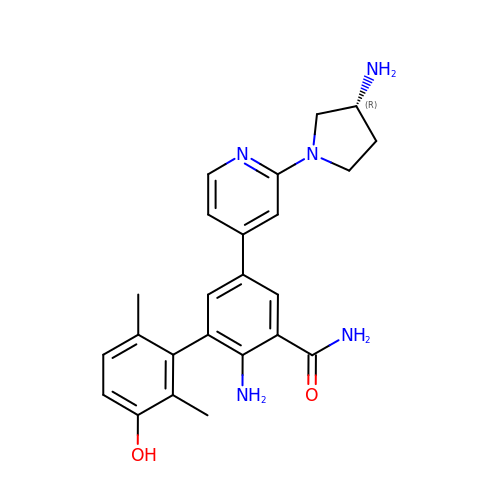2-azanyl-5-[2-[(3~{R})-3-azanylpyrrolidin-1-yl]pyridin-4-yl]-3-(2,6-dimethyl-3-oxidanyl-phenyl)benzamide | C24 H27 N5 O2 | OVPMEUICXCKOJF-QGZVFWFLSA-N>[2x]AKPDRSSFVPSLFSKKKKNVTMRSIKTTRDRVPTYQYNMNFEKLGKCIIINNKNFDKVTGMGVRNGTDKDAEALFKCFRSLGFDVIVYNDCSCAKMQDLLKKASEEDHTNAACFACILLSHGEENVIYGKDGVTPIKDLTAHFRGDRCKTLLEKPKLFFIQACRGTELDDGIQADSGPINDTDANPRYKIPVEADFLFAYSTVPGYYSWRSPGRGSWFVQALCSILEEHGKDLEIMQILTRVNDRV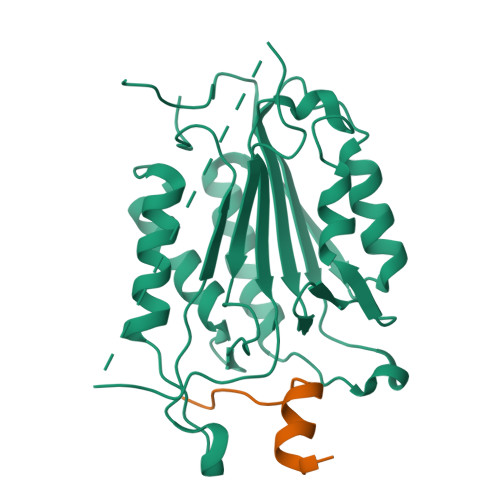ARHFESQSDDPHFHEKKQIPCVVSMLTKELYFSQ;>[2x]YLGSRDHFALDRPSETHADYLLRTGQVVDISDTIYPRNPAMYSEEARLKSFQNWPDYAHLTPRELASAGLYYTGIGDQVQCFCCGGKLKNWEPCDRAWSEHRRHFPNCFFVLGRNLNIRSESDAVSSDRNFPNSTNLPRNP> MSSQIRQNYSTDVEAAVNSLVNLYLQASYTYLSLGFYFDRDDVALEGVSHFFRELAEEKREGYERLLKMQNQRGGRALFQDIKKPAEDEWGKT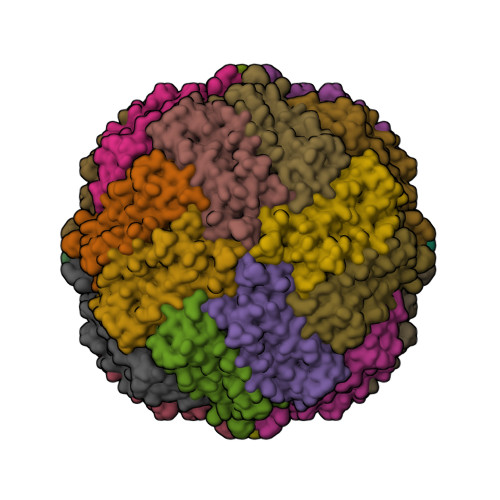PDAMKAAMALEKKLNQALLDLHALGSARTDPHLCDFLETHFLDEEVKLIKKMGDHLTNLHRLGGPEAGLGEYLFERLTLKHD The enzyme porphobilinogen deaminase (PBGD; hydroxymethylbilane synthase; EC 2.5.1.61) catalyses an early step of the tetrapyrrole-biosynthesis pathway in which four molecules of the monopyrrole porphobilinogen are condensed to form a linear tetrapyrrole. The enzyme possesses a dipyrromethane cofactor, which is covalently linked by a thioether bridge to an invariant cysteine residue (Cys241 in the Bacillus megaterium enzyme). The cofactor is extended during the reaction by the sequential addition of the four substrate molecules, which are released as a linear tetrapyrrole product. All enzymes in this family adopt a three-domain fold in which domains 1 and 2 resemble the fold of type II periplasmic binding proteins and the third domain, to which the cofactor is covalently attached, adopts a distinct α+β topology.

In addition, the structure of the enzyme in which the cofactor has undergone more extensive oxidation is presented at the slightly lower resolution of 1.6 Å with similar refinement and validation statistics. The collection of data from two crystals, which were flash-cooled at periods of 40 and 50 d after purification, demonstrates that the dipyrromethane cofactor adopts two conformations corresponding to partially oxidized states. Accordingly, refinement of the occupancies of the oxidized and reduced states in the two structures reported here showed that the proportion of the oxidized dipyrromethanone form increases in a time-dependent manner from 30% in the case of the 40-day-old protein to 50% for the 50-­day-old protein. In both of the structures of B. megaterium PBGD that we report here, the C2 ring clearly adopts two positions, one of which corresponds to the fully reduced dipyrromethane that has been observed in structures of the E. coli and human enzymes when they are crystallized under reducing conditions. In the B. megaterium enzyme the electron-density map clearly shows that the oxidized conformation of the cofactor has the same oxygen substituent in the C2 ring, which is suggestive of the same dipyromethenone form. However, the other α-position of the C2 ring which partakes in the methylene bridge with the adjacent C1 pyrrole is clearly tetrahedral, in contrast to the trigonal planar configuration that is found in dipyrromethenone. The two structures reported here superimpose very closely, with an r.m.s.d. of only 0.17 Å for all Cα atoms. Interestingly, domains 2 and 3 appear to rotate towards domain 1 by approximately 0.6° in the more oxidized structure, suggesting that as the proportion of cofactor in the more extended state increases, the active site of the enzyme is able to close more. This rigid-body rotation gives rise to movements of several loops over the active site of at most 0.5 Å.

> SHMRKIIVGSRRSKLALTQTKWVIEQLKKQGLPFEFEIKEMVTKGDQILNVTLSKVGGKGLFVKEIEQAMLDKEIDMAVHSMKDMPAVLPEGLTIGCIPLREDHRDALISKNGERFEELPSGAVIGTSSLRRGAQLLSMRSDIEIKWIRGNIDTRLEKLKNEDYDAIILAAAGLSRMGWSKDTVTQYLEPEISVPAVGQGALAIECRENDHELLSLLQALNHDETARAVRAERVFLKEMEGGCQVPIAGYGRILDGGNIELTSLVASPDGKTIYKEHITGKDPIAIGSEAAERLTSQGAKLLIDRVKEELDK> MHLNPAEKEKLQIFLASELLLRRKARGLKLNYPEAVAIITSFIMEGARDGKTVAMLMEEGKHVLTRDDVMEGVP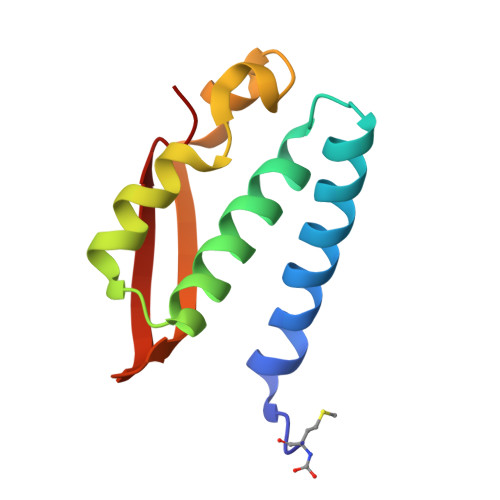EMIDDIQAEATFPDGTKLVTVHNPIS> MEWIQSLPKIELHAHLNGSIRDSTLLELARVLGEKGVIVFADVEHVIQKNDRSLVEVFKLFDLIHKLTTDHKTVTRITREVVEDFALENVVYLELRTTPKRSDSIGMSKRSYMEAVIQGLRSVSEVDIDFVTASDSQKLHNAGDGIGRKKIYVRLLLSIDRRETTESAMETVKLALEMRDVGVVGIDLSGNPLVGEWSTFLPALQYAKDNDLHITLHCG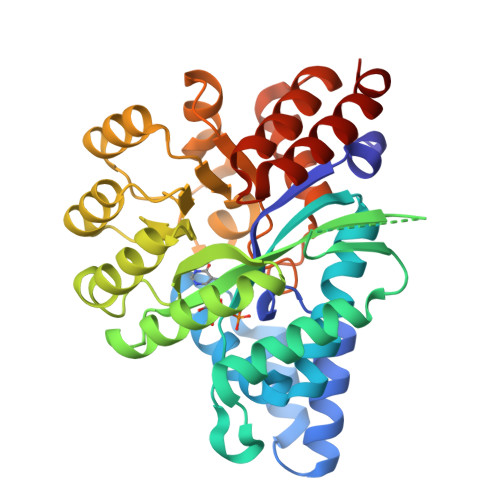EVPNPKEIQAMLDFKPHRIGHACFFKDEDWTKLKSFRIPVEICLTSNIVTKSISSIDIHHFADLYNAKHPLILCTNDFGVFSTSLSNEYALAVRSLGLSKSETFALARAAIDATFAEDEVKQQLRFIFDSASPEHV> MAPKAKIVLVGSGMIGGVMATLIVQKNLGDVVLFDIVKNMPHGKALDTSHTNVMAYSNCKVSGSNTYDDLAGSDVVIVTAGFTKAPGKSDKEWNRLDLLPLNNKIMIEIGGHIKKNCPNAFIIVVTNPVDVMVQLLHQHSGVPKNKIIGLGGVLDTSRLKYYISQKLNVCPRDVNAHIVGAHGNKMVLLKRYITVGGIPLQEFINNKLISDAELEAIFDRTVNTALEIVN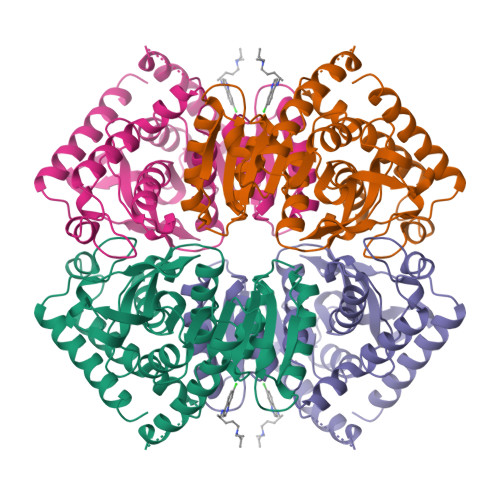LHASPYVAPAAAIIEMAESYLKDLKKVLICSTLLEGQYGHSDIFGGTPVVLGANGVEQVIELQLNSEEKAKFDEAIAETKRMKALA>[2x]SNALNSAPTPRDVVANAPAPVQAAVAGAQEYAAQAGLNTEELAVDALYNAIKVRLAG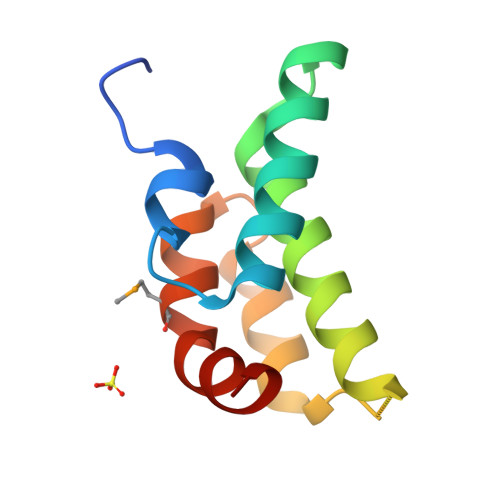TGLGIPPQIEAFYQANRTNFNGFYMANRGAIDFIFSM>MSAKAISEQTGKELLYKFICTTSAIQNRFKYARVTPDTDWARLLQDHPWLLSQNLVVKPDQLIKRRGKLGLVGVNLTLDGVKSWLKPRLGQEATVGKATGFLKNFLIEPFVPHSQAEEFYVCIYATREGDYVLFHHEGGVDVGDVDAKAQKLLVGVDEKLNPEDIKKHLLVHAPEDKKEILASFISGLFNFYEDLYFTYLEINPLVVTKDGVYVLDLAAKVDATADYICKVKWGDIEFPPPFGREAYPEEAYIADLDAKSGASLKLTLLNPKGRIWTMVAGGGASVVYSDTICDLGGVNELANYGEYSGAPSEQQTYDYAKTILSLMTREKHPDGKILIIGGSIANFTNVAATFKGIVRAIRDYQGPLKEHEVTIFVRRGGPNYQEGLRVMGEVGKTTGIPIHVFGTETH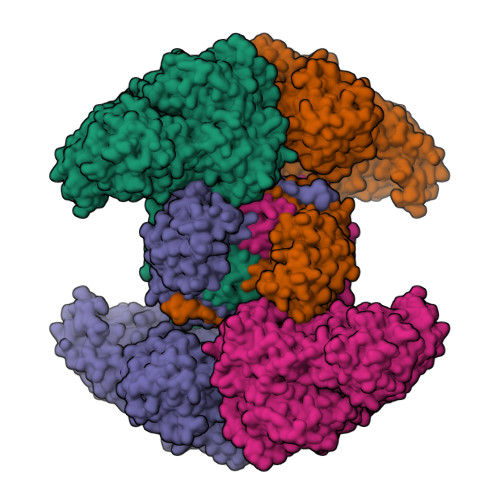MTAIVGMALGHRPIPNQPPTAAHTANFLLNASGSTSTPAPSRTASFSESRADEVAPAKKAKPAMPQDSVPSPRSLQGKSTTLFSRHTKAIVWGMQTRAVQGMLDFDYVCSRDEPSVAAMVYPFTGDHKQKFYWGHKEILIPVFKNMADAMRKHPEVDVLINFASLRSAYDSTMETMNYAQIRTIAIIAEGIPEALTRKLIKKADQKGVTIIGPATVGGIKPGCFKIGNTGGMLDNILASKLYRPGSVAYVSRSGGMSNELNNIISRTTDGVYEGVAIGGDRYPGSTFMDHVLRYQDTPGVKMIVVLGEIGGTEEYKICRGIKEGRLTKPIVCWCIGTCATMFSSEVQFGHAGACANQASETAVAKNQALKEAGVFVPRSFDELGEIIQSVYEDLVANGVIVPAQEVPPPTVPMDYSWARELGLIRKPASFMTSICDERGQELIYAGMPITEVFKEEMGIGGVLGLLWFQKRLPKYSCQFIEMCLMVTADHGPAVSGAHNTIICARAGKDLVSSLTSGLLTIGDRFGGALDAAAKMFSKAFDSGIIPMEFVNKMKKEGKLIMGIGHRVKSINNPDMRVQILKDYVRQHFPATPLLDYALEVEKITTSKKPNLILNVDGLIGVAFVDMLRNCGSFTREEADEYIDIGALNGIFVLGRSMGFIGHYLDQKRLKQGLYRHPWDDISYVLPEHMSMKLAAALEHHHHHHHH[4x]1-(5-~{tert}-butyl-2-quinolin-6-yl-pyrazol-3-yl)-3-[3-(4-morpholin-4-yl-7~{H}-pyrrolo[2,3-d]pyrimidin-5-yl)phenyl]urea | C33 H33 N9 O2 | 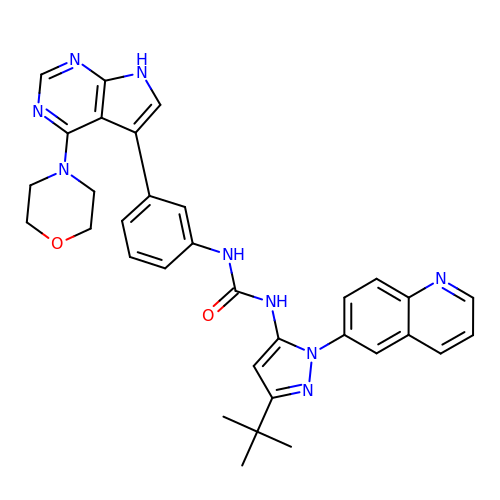VZYRIZGYTGKYQV-UHFFFAOYSA-N>[2x]MESCYNPGLDGIIEYDDFKLNSSIVEPKEPAPETADGPYLVIVEQPKQRGFRFRYGCEGPSHGGLPGASSEKGRKTYPTVKICNYEGPAKIEVDLVTHSDPPRAHAHSLVGKQCSELGICAVSVGPKDMTAQFNNLGVLHVTKKNMMGTMIQKLQRQRLRSRPQGLTEAEQRELEQEAKELKKVMDLSIVRLRFSAFLRASDGSFSLPLKPVISQPIHDSKSPGASNLKISRMDKTAGSVRGGDEVYLLCDKVQKDDIEVRFYEDDENGWQAFGDFSPTDVHKQYAIVFRTPPYHKMKIERPVTVFLQLKRKRGGDVSDSKQFTYYP

Mammalian NF-κB is assembled combinatorially from five subunits, p50/NF-κB1, p52/NF-κB2, RelA/p65, c-Rel, and RelB, into homo- and heterodimers which bind to specific DNA sequences, known as κB site or κB DNA. The DD alone mediates protein homo- and heterodimerization; the NTD and DD together are responsible for DNA binding; and the NLS region is flexible in solution and together with the DD forms the binding sites for the inhibitor of NF-κB (IκB) proteins. The mammalian NF-κB p52:p52 homodimer together with its cofactor Bcl3 activates transcription of κB sites with a central G/C base pair (bp), while it is inactive toward κB sites with a central A/T bp. The p50 and p52 subunits bind to a 5 bp half-site (5′-GGGNN-3′), while the RelA and c-Rel subunits prefer a 4 bp half-site (5′-NNCC-3′).

To test if the DNA and protein length variations induce structural changes in the complex, we set out to co-crystallizations of a shorter p52 protein (aa 1–327) with all three PSel-κB DNAs at various lengths. This short p52 protein only co-crystallized with a 13 bp PSel (mutant A/T-centric) DNA but not the (natural G/C-centric) or (−1/+1 swap) DNAs in any lengths. The conformation of this complex is nearly identical to p52-MHC-κB complex with minor groove width less than 4 Å at the central position. This crystal with short p52 is in a different crystal form compared to the three structures with the long p52, and it is also in a different crystal form compared to the MHC-κB DNA complex, suggesting that crystal packing is unlikely to be the main cause of the structural differences, and that both the DNA and protein lengths play significant roles. Therefore, we observed an influence of the length of the p52 protein on the conformation of the κB DNA and the organization of the p52:p52 dimer in the complex. The same Arg52 in the complex with the short 13 bp PSel (mutant A/T-centric) or the MHC-κB DNA only hydrogen bonds with the O6 group, but not the N7, of G at ±3. In addition, Ser61 also makes direct contact with A at ±6 and ±7 positions; these contacts are not possible for the short p52 (aa 1–327) co-crystallized with 13 bp κB DNAs such as MHC and PSel (mutant A/T-centric)-κB. p52 monomer II makes contact with only three G(s) from position −3 to −5 (right). Interestingly, all other NF-κB-DNA complexes, including the short p52:p52 homodimer bound to both 13 bp MHC-κB and PSel (mutant A/T-centric)-κB DNAs, exhibit more backbone contacts by Gln284 and Gln254. The short p52 protein (aa 1–327) failed to interact with Bcl3, partly due to the lack of the GRR.>[4x]MDSTKAQTPEEQRAKNAKTILENIQIYERMCDLFGVSEDDKLIIENSISIERMIRVVTDKKYQDKKLKNAGSDLEKIANAGKVFCRLVESTAGKCSARLGMALKPNVEAVLTDVLGNELDRAAVLGKRMGFTAMFKSNLEEVLYQRGKNQLKKRNSAETFTLSQGASLEARFRPIMEKHLGVGTVVASIKNILASKKNGNYKNKMVRKPGGNRESWSPLEREISFLNKKLFPGPMRQLCKKFEYLNDQEKQLALNLMLDASLILKPQVTHKMIMPWSMWLAVKKYAEMNKGSPSLEDLAAYSGVRAFMAFNTACYMSKFTIGKGIVGDAEIMENGNDKMQILAMACFGLAYEDTGIVAAMISQPMKKRYQLKVGNFNPPEEGTIKGTSAGYFHKWAEFGNRLPFNSFGTGESKQISNSGVFAVQRPSTTNIQRLAELMARNTGETSDNFTQLVQKIREQVGTFADQKANLREFTGGYIYDITDVTKSNPKIPQLGGNSFFFEFTGSDVPRTGAKRRVGGADDVTLGTSQPKKRGRQGAGVESSMDIETVGED

All these results suggested it was a new genus of the Orthomyxoviridae, temporarily named C/swine/Oklahoma/1334/2011 (C/swine/OK) and then Influenza D virus (IDV). In this paper, we characterized D/NP and solved the X-ray structure of its tetramer. We demonstrated that the C-terminal D/NPTAIL presents all the characteristics of an intrinsically disordered protein and that is involved in the nuclear import through its interaction with cellular importins-α.

Full length D/NP was crystallized in sodium malonate as small fine needles that diffract X-rays up to 2.4 Å resolution. The structure was solved by molecular replacement using a starting model of the monomer of the A/NP R416A mutant. The molecular replacement using the tetrameric B/NP model did not give any acceptable solutions. The asymmetric unit contained four molecules arranged as a tetramer (Fig. 2a and refinement statistics in Supplementary Table 1), consistent with the observations made by electron microscopy. Based on the electron density, 87% of the model could be built, from residues 8 to 514. Several internal loops were missing and the C-terminal 50 residues were disordered. The oligomerization-loop of one protomer plugged into a cavity of its neighbour. The loop was then stabilized by several kind of contacts; mainly hydrophobic (by the side chain of the strictly conserved Phe-421 and Val-423) and of several aromatic residues lying in the pocket of the neighbouring monomer but also the salt bridge between an arginine from one monomer (Arg-425) interacting with a glutamate of the neighbour (Glu-352). The overall folds of A/NP, B/NP, ISA/NP and D/NP were very similar with root-mean-square deviations (rmsd) between 1.6 Å (for 383 Cα for the comparison A/NP with B/NP) and 2.9 Å (for 340 Cα for the comparison D/NP with ISA/NP). Twenty or 71 residues without any structure are found N-terminally before the cores of A/ and B/NP whereas for D/NP, the core starts with a very short version of an N-terminal tail (only 7 residues), which seems to be compensated by the presence of a carboxy-terminal NPTAIL of 51 residues. The sequence analysis of D/NP showed no import signals in its N-terminal part but suggested the presence of a bipartite NLS within D/NPTAIL (514KRR-X14-KKRGR535).4-[2-(5-methyl-1-naphthalen-2-yl-pyrazol-3-yl)oxyethyl]morpholine 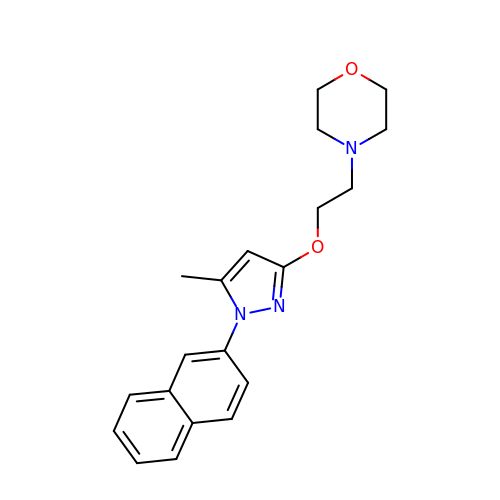| C20 H23 N3 O2 | DGPGXHRHNRYVDH-UHFFFAOYSA-N> EEIRPKEVYLDRKLLTLEDKELGSGNFGTVKKGYYQMKKVVKTVAVKILKNEANDPALKDELLAEANVMQQLDNPYIVRMIGICEAESWMLVMEMAELGPLNKYLQQNRHVKDKNIIELVHQVSMGMKYLEESNFVHRDLAARNVLLVTQHYAKISDFGLSKALRADENYYKAQTHGKWPVKWYAPECINYYKFSSKSDVWSFGVL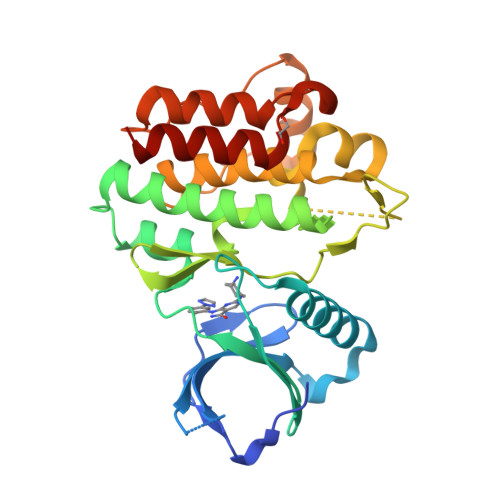MWEAFSYGQKPYRGMKGSEVTAMLEKGERMGCPAGCPREMYDLMNLCWTYDVENRPGFAAVELRLRNYYYDVVN> GHMRELQADFVKPARIDILLDMPPASRDLQLKHSWNSEDRSLNIFVKEDDKLTFHRHPVAQSTDCIRGK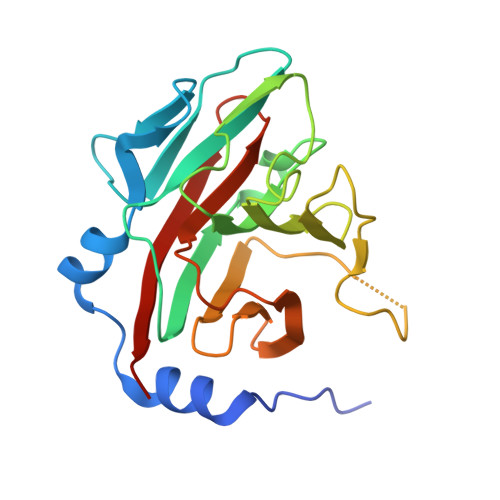VGLTKGLHIWEIYWPTRQRGTHAVVGVCTADAPLHSVGYQSLVGSTEQSWGWDLGRNKLYHDSKNCAGVTYPAILKNDEAFLVPDKFLVALDMDEGTLSFIVDQQYLGIAFRGLRGKKLYPIVSAVWGHCEITMRYIGGLVDELN Different AAF variants are expressed by different EAEC strains, where they are required for the bacterium's adherence to small and large intestinal mucosa. As with Afa/Dr polyadhesins, AAF consist of two secreted protein subunits, a major subunit (A) and a putative minor subunit (B). In the fiber, subunits are linked together by donor strand complementation (DSC) with an N-terminal Gd donor strand segment of one subunit inserted into the hydrophobic cleft of a neighboring subunit. In this study, we report X-ray crystallographic and NMR studies of monomeric, donor-strand-complemented major and minor subunits of AAF/I from the German outbreak strain and AAF/II from EAEC strain 042 and provide an atomic resolution model for the structure of the entire fimbriae.

The DSC-monomers of the major subunits (AggAdsA and AafAdsA) have a classical Ig-like fold that consists of two β sheets packed against each other in a β sandwich. Instead, it has additional strands C and D, which form the edge of β sheet 2 (CDC1C2FGdA2) in this subunit. Both strand F and the donor strand (Gd) at the other edge of sheet 2 are longer in AggAdsA than in AafAdsA. The donor strand of AggAdsA inserts seven classical donor residues in to the acceptor cleft, which is two more than AafAdsA and other structurally characterized subunits from FGL CU systems. In addition, AggAdsA contains an α helix in the loop between B and C1 strands, which is absent in AafAdsA. These features give AggAdsA a more elongated shape than AafAdsA. To examine if fibronectin is a common receptor for AAF, we studied AggAdsA-fibronectin interactions using surface plasmon resonance (SPR). The experiment revealed specific binding with a dissociation constant of 16±2 µM. We focused the mutagenesis on surface patches comprising proximal pairs of lysines (including Lys51 and Lys109, Lys55 and Lys103, and Lys73 and Lys76) and the three closely positioned lysines Lys73, Lys76, and Lys78. All the double mutants exhibited significant decreases in fibronectin binding and, despite the absence of the cooperatively expected for a polymeric AggA fiber, the affinity for the triple mutant of monomeric AggAdsA dropped below the detection limit of the experiment. The pocket is particularly well pronounced in AAF/I. Three closely positioned lysines (73, 76 and 78), mutations of which practically abolished the binding, are located in the loop between the C2 and Ć strands at the bottom of the subunit.

>ASQHHHHHHVTNDCPVTITTTPPQTVGVSSTTPIGFSAKVTTSDQCIKAGAKVWLWGTGPANKWVLQHAKVAKQKYTLNPSIDGGADFVNQGTDAKIYKKLTSGNKFLNASVSVNPKTQVLIPGEYTMILHAAVDFDNKQGGASQQTTQTIRLTVT[2x]>[3x]CVIFPVEIDVSQTIIRDCQVDKQTRELVYINKIMNTQLTKPVLMMFNISGPIRSVTRKNNNLRDRIKSKVDEQFDQLERDYSDQMDGFHDSIKYFKDEHYSVSCQNGSVLKSKFAKILKSHDYTDKKSIEAYEKYCLPKLVDER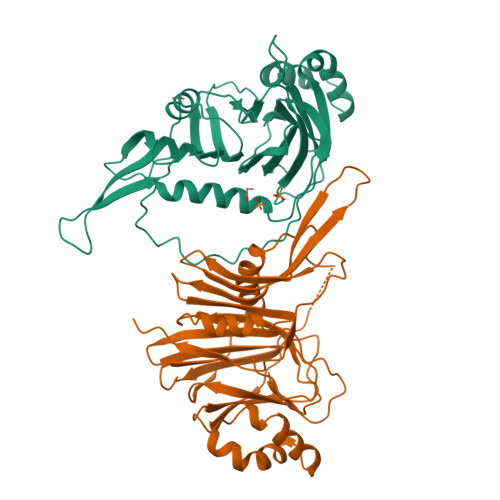NDYYVAVCVLKPGFENGSNQVLSFEYNPIGNKVIVPFAHEINDTGLYEYDVVAYVDSVQFDGEQFEEFVQSLILPSSFKNSEKVLYYNEASKNKSMIYKALEFTTESSWGKSEKYNWKIFCNGFIYDKKSKVLYVKLHNVTSALNKNVILNTIKA> MHRPEAEKWLRRFERAPDARARLVCLPHAGGSASFFFPLAKALAPAVEVLAVQYPGRQDRRHEPPVDSIGGLTNRLLEVLRPFGDRPLALF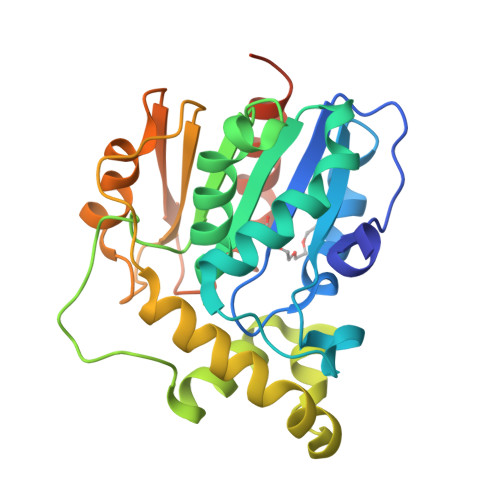GHAMGAIIGYELALRMPEAGLPAPVHLFASGRRAPSRYRDDDVRGASDERLVAELRKLGGSDAAMLADPELLAMVLPAIRSDYRAVETYRHEPGRRVDCPVTVFTGDHDPRVSVGEARAWEEHTTGPADLRVLPGGHFFLVDQAAPMIATMTEKLAGPALTGSTGGNSLEHHHHHH> AIRNCIIGKGRSYKGTVSITKSGIKCQPWSSMIPHEHSFLPSSYRGKDLQENYCRNPRGEEGGPWCFTSNPEVRYEVCDIPQCSEVECIIGKGRSYKGTVSITKSGIKCQPWSSMIPHEHSFLPSSYRGKDLQENYC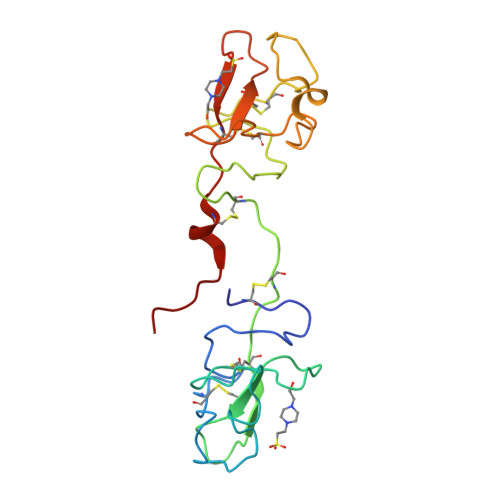RNPRGEEGGPWCFTSNPEVRYEVCDIPQCSEVEHHHHHH> GGLAALTKPPTFATVEAERAWLKERLVAAIRIFANEGFDHTVAGHLTVRDPENKHHFWVNPFGLAFRLMTVSDLILVNQEGTVIGGGKEGRRIVNLAGFMIHSAIHKARPEVQAICHSHSTYGKAFSSLGKPLAITTQDSCAFYGDVALLGDFGGVVIEEKESGTIAVALQQKKAIILQNHGLLTVGTTID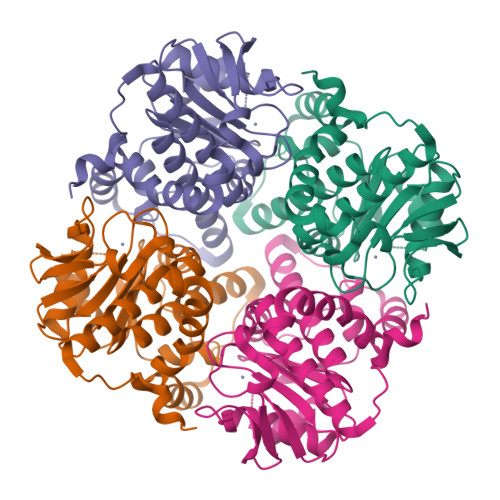SAVAWFIMLEKQCQVQLLADAAGQTIPIDEPQAAFTFKELGHEQAGYFQASPYFQVIEHLQGEEYRK> MGSDTLAAPPHGAPRVDRDMVSRFATCCRALGLTVNDRQRPADLTAARAGFAGLTHLAHDQCDAWIGLAAAGEVTPAVVDAVWRTVASAGVLQREIGLAAGELGFTYDTGWYLQFRATEPDDFQLAYAARLYEAGEFGEADGLVGEILARRPGWFDARWLQVAINHRAQRWSDVVRLLTPVVTLPSLDDVTSHAVRTALGISLARLGMFAPAMSY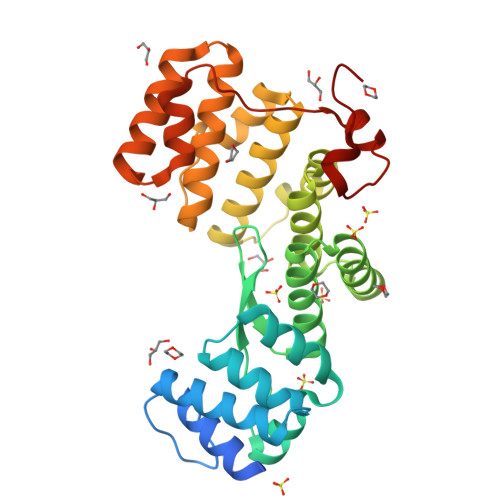LEDPAGPIEVAAVDGALAKALTLRAQGEDDEATEVLQDLFATHPENTQVEQALLDTSFGLVTTTSARIEARSDPWDPETEPSEAE> MALIDDFKARFPNLDGSLVDALVPVYENNYSCYYGGSYENDCDKEAILLLIAHLVVTDPSYSGDESSSRAVASQSVGSVSVSFVAGSTGSDWTNWLNSTRYGQLFLMVTSNNMG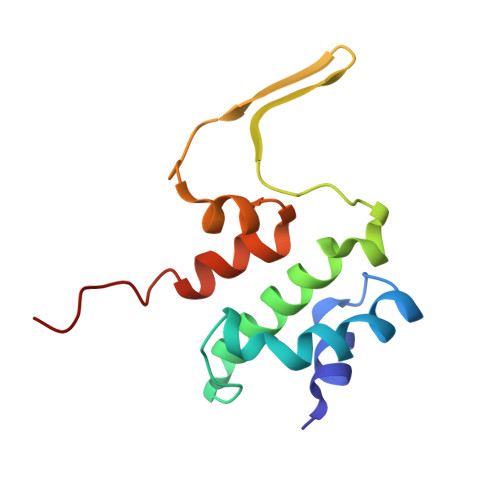PSFA>[2x]ILPDSVDWREKGCVTEVKYQGSCGASWAFSAVGALEAQLKLKTGKLVSLSAQNLVDCSTEKYGNKGCNGGFMTTAFQYIIDNKG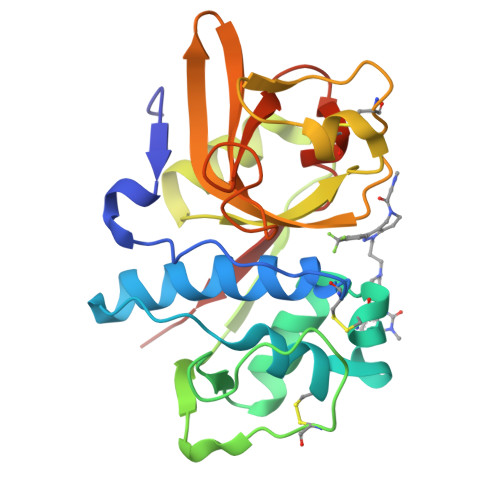IDSDASYPYKAMDQKCQYDSKYRAATCSKYTELPYGREDVLKEAVANKGPVSVGVDARHPSFFLYRSGVYYEPSCTQNVNHGVLVVGYGDLNGKEYWLVKNSWGHNFGEEGYIRMARNKGNHCGIASFPSYPEILQGGG>GHMAIAPNTRVLVAGYGLPAEFCVTTLIGMGVEIDKIAVATHREDNRNCGLHSMLRLRNIQFTTAAANSEEFYEFGANFAPDMIISMHYRSLIPGRFLKLAKKGSVNLHPSLLPAYRGTNSVAWVIINGESETGFSYHRMDENADTGAILLQERISVEETDTAFSLFHRQIARAMLRLEEVILKLDQGDPGFAQLGEASYYARELPFG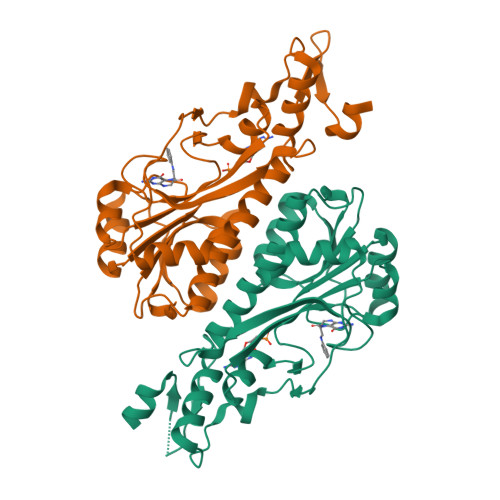GVIDPRWSEVQIDRFIRAMFFPPFPPAVLKIDGKVYYVPSIDIYRSLMRGIPS[4x]> MDDMQVYIANLGKYNEGELVGA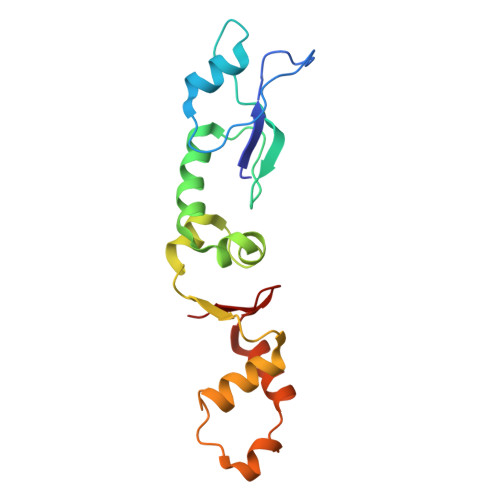WFTFPIDFEEVKEKIGLNDEYEEYAIHDYELPFTVDEYTSIGELNRLWEMVSELPEELQSELSALLTHFSSIEELSEHQEDIIIHSDCDDMYDVARYYIEETGALGEVPASLQNYIDYQAYGRDLDLSGTFISTNHGIFEIVY>MSRAKAAPVAGPEVAANRAGRQARIVAILSSAQVRSQNELAALLAAEGIEVTQATLSRDLEELGAVKLRGADGGTGIYVVPEDGSPVRGVSGGTDRMARLLGELLVSTDDSGNLAVLRTPPGAAHYLASAIDRAALPQVVGTIAGDDTILVVAR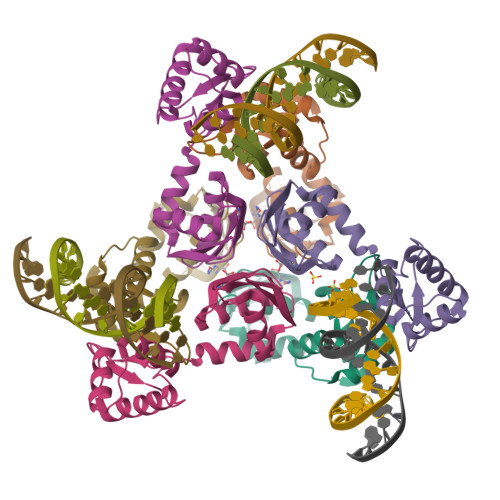EPTTGAQLAGMFENLR[6x]>MFSKLAHLQRFAVLSRGVHSSVASATSVATKKTVQGPPTSDDIFEREYKYGAHNAHPLPVALERGKGIYLWDVEGRKYFDFLSSISAVNQGHCHPKIVNALKSQVDKLTLTSRAFYNNVLGEYEEYIT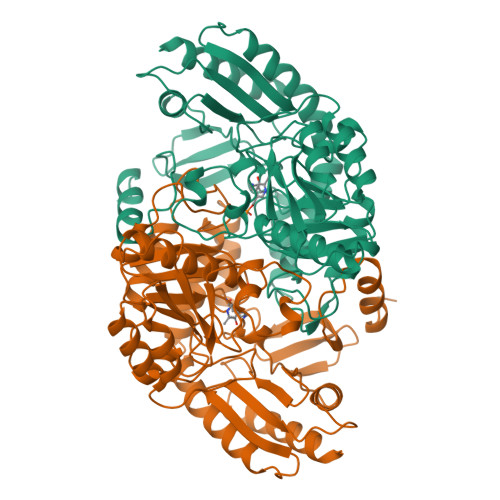KLFNYHKVLPMNTGVEAGETACKLARKWGYTVKGIQKYKAKIVFAAGNFWGRTLSAISSSTDPTSYDGFGPFMPGFDIIPYNDLPALERALQDPNVAAFMVEPIQGEAGVVVPDPGYLMGVRELCTRHQVLFIADEIQTGLARTGRWLAVDYENVRPDIVLLGKALSGGLYPVSAVLCDDDIMLTIKPGEHFSTYGGNPLGCRVAIAALEVLEEENLAENADKLGIILRNELMKLPSDVVTAVRGKGLLNAIVIKETKDWDAWKVCLRLRDNGLLAKPTHGDIIRFAPPLVIKEDELRESIEIINKTILSF[3x]> MAAQRRSLLQSEQQPSWTDDLPLCHLSGVGSASNRSYSADGKGTESHPPEDSWLKFRSENNCFLYGVFNGYDGNRVTNFVAQRLSAE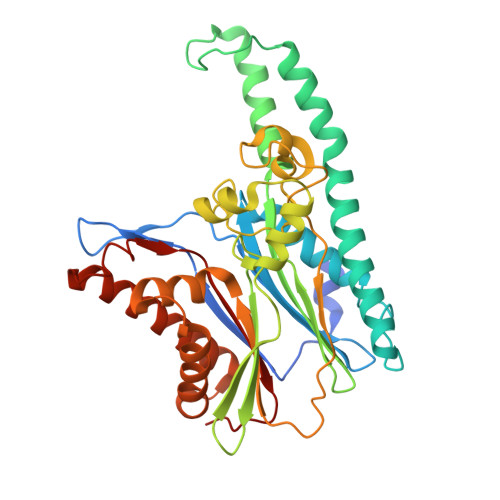LLLGQLNAEHAEADVRRVLLQAFDVVERSFLESIDDALAEKASLQSQLPEGVPQHQLPPQYQKILERLKTLEREISGGAMAVVAVLLNNKLYVANVGTNRALLCKSTVDGLQVTQLNVDHTTENEDELFRLSQLGLDAGKIKQVGIICGQESTRRIGDYKVKYGYTDIDLLSAAKSKPIIAEPEIHGAQPLDGVTGFLVLMSEGLYKALEAAHGPGQANQEIAAMIDTEFAKQTSLDAVAQAVVDRVKRIHSDTFASGGERARFCPRHEDMTLLVRNFGYPLG>[3x]GPCGASEVVTSGQKIAVPAASHHFCFSVDLRSVHDLELSFPV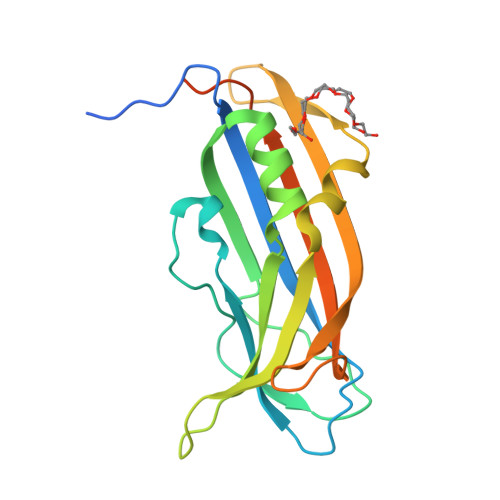NCILRYSYPFFGSAAPIMTNPPVEVRKNMEVFLPQSYCAFDFATMPHQLQDTFLRIPLLVELWHKDKMSKDLLLGVARIQLSNILSSEKTRFLGANGEQCWRQTYSESVPVIAAQGSNNRILDLSYTMTLEDYGLVKMREIFVSESSQGVPAVDQKPSS> GSHMSGKARLHYPVTRQGEQVDHYFGQAVADPYRWLEDDRSPETEAWVKAQNAVTQDYLAQIPYRAAIKEKLAASWNYAKEGAPFWWGRYHYFFKNDGLQNQNVLWRQQEGKPAEVFLDPNTLSPDGTTALDQLSFSRDGRILAYSLSLAGSDWREIHLMDVESKQPLETPLKDVKFSGISWLGNEGFFYSSYDKPDGSELSARTDQHKVYFHRLGTAQEDDRLVFGAIPAQHHRYVGATVTEDQRFLLISAANSTSGNRLYVKDLSQENAPLLTVQGDLDADVSLVDNKGSTLYLLTNRDAPNRRLVTVDAANPGPAHWRDLIPERQQVLTV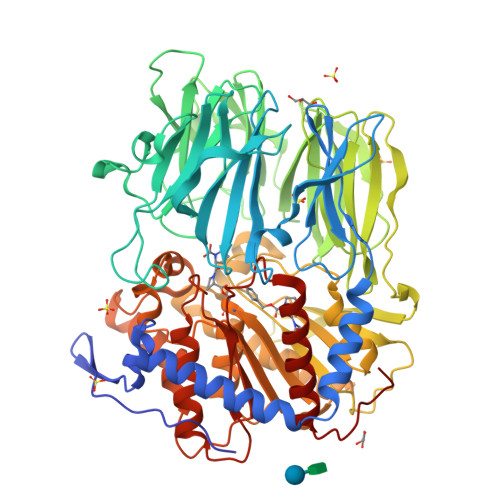HSGSGYLFAEYMVDATARVEQFDYEGKRVREVALPGLGSVSGFNGYWWDPALYFGFENYAQPPTLYRFEPKSGAISLYRASAAPFKPEDYVSEQRFYQSKDGTRVPLIISYRKGLKLDGSNPTILYGYGGFDVSLTPSFSVSVANWLDLGGVYAVANLRGGGEYGQAWHLAGTQQNKQNVFDDFIAAAEYLKAEGYTRTDRLAIRGGSNGGLLVGAVMTQRPDLMRVALPAVGVLDMLRYHTFTAGTGWAYDYGTSADSEAMFDYLKGYSPLHNVRPGVSYPSTMVTTADHDDRVVPAHSFKFAATLQADNAGPHPQLIRIETNAGHGAGTPVAKLIEQSADIYAFTLYEMGYRELPRQP> GHMKEEEMKRFCKAQTIQRRLNEIEAALRELEAE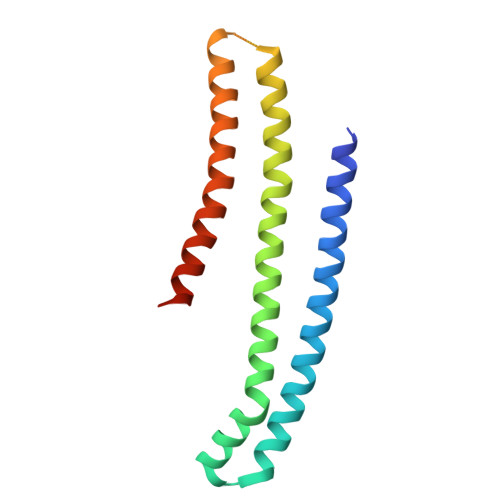GVKLELALRRQSSSPEQQKKLWVGQLLQLVDKKNSLVAEEAELMITVQELNLEEKQWQLDQELRGYMNREENLKTAADRQAEDQVLRKLVDLVNQRDALIRFQEERRLSELALGTGAQG> SASEEQVAQDTEEVF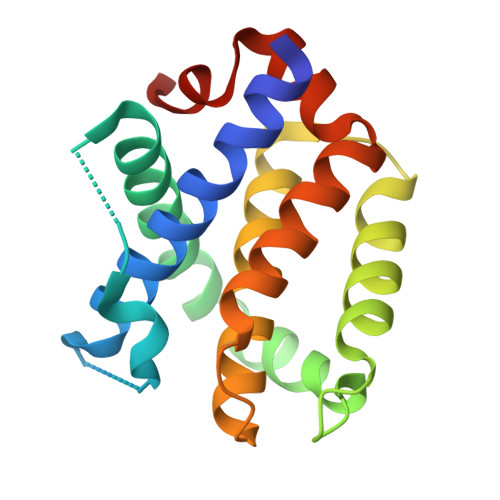RSYVFYRHQQEQEAEGVAAPADPEMVTLPLQPSSTMGQVGRQLAIIGDDINRRYDSEFQTMLQHLQPTAENAYEYFTKIATSLFESGINWGRVVALLGFGYRLALHVYQHGLTGFLGQVTRFVVDFMLHHSIARWIAQRGGWVAALNLCNG>MTSPQLEWTLQTLLEQLNEDELKSFKSLLWAFPLEDVLQKTPWSEVEEADGKKLAEILVNTSSENWIRNATVNILEEMNLTELCKMAKAEMMEDGQVQEIDNPELGDAEEDSELAKPGEKEGWRNSMEKQSLVWKNTFWQGDIDNFHDDVTLRNQRFIPFLNPRTPRKLTPYTVVLHGPAGVGKTTLAKKCMLDWTDCNLSPTLRYAFYLSCKELSRMGPCSFAELISKDWPELQDDIPSILAQAQRILFVVDGLDELKVPPGALIQDICGDWEKKKPVPVLLGSLLKRKMLPRAALLVTTRPRALRDLQLLAQQPIYVRVEGFLEEDRRAYFLRHFGDEDQAMRAFELMRSNAALFQLGSAPAVCWIVCTTLKLQMEKGEDPVPTCLTRTGLFLRFLCSRFPQGAQLRGALRTLSLLAAQGLWAQMSVFHREDLERLGVQESDLRLFLDGDILRQDRVSKGCYSFIHLSFQQFLTALFYALEKEEGEDRDGHAWDIGDVQKLLSGEERLKNPDLIQVGHFLFGLANEKRAKELEATFGCRMSPDIKQELLQCKAHLHANKPLSVTDLKEVLGCLYESQEEELAKVVVAPFKEISIHLTNTSEVMHCSFSLKHCQDLQKLSLQVAKGVFLENYMDFELDIEFERCTYLTIPNWARQDLRSLRLWTDFCSLFSSNSNLKFLEVKQSFLSDSSVRILCDHVTRSTCHLQKVEIKNVTPDTAYRDFCLAFIGKKTLTHLTLAGHIEWERTMMLMLCDLLRNHKCNLQYLRLGGHCATPEQWAEFFYVLKANQSLKHLRLSANVLLDEGAMLLYKTMTRPKHFLQMLSLENCRLTEASCKDLAAVLVVSKKLTHLCLAKNPIGDTGVKFLCEGLSYPDCKLQTLVLQQCSITKLGCRYLSEALQEACSLTNLDLSINQIARGLWILCQALENPNCNLKHLRLWSCSLMPFYCQHLGSALLSNQKLETLDLGQNHLWKSGIIKLFGVLRQRTGSLKILRLKTYETNLEIKKLLEEVKEKNPKLTIDCN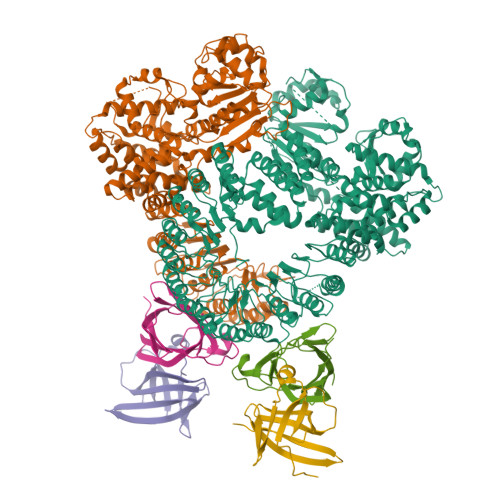ASGATAPPCCDFFC[2x];>EAVTDHPDRLWAWEKFVYLDEKQHAWLPLTIEIKDRLQLRVLLRREDVVLGRPMTPTQIGPSLLPIMWQLYPDGRYRSSDSSFWRLVYHIKIDGVEDMLLELLPDD[4x]>GPLGSVAAQKKKAQDEYGAASITILEGLEAVRKRPGMYIGSTGERGLHHLIWEVVDNAVDEAMAGYATTVNVVLLEDGGVEVADDGRGIPVATHASGIPTVDVVMTQLHAGGKFDSDAYAISGGLHGVGVSVVNALSTRLEVEIKRDGYEWSQVYEKSEPLGLKQGAPTKKTGSTVRFWADPAVFETTEYDFETVARRLQEMAFLNKGLTINLTDERVTQDEVVDEVVSDVAEAPKSASERAAESTAP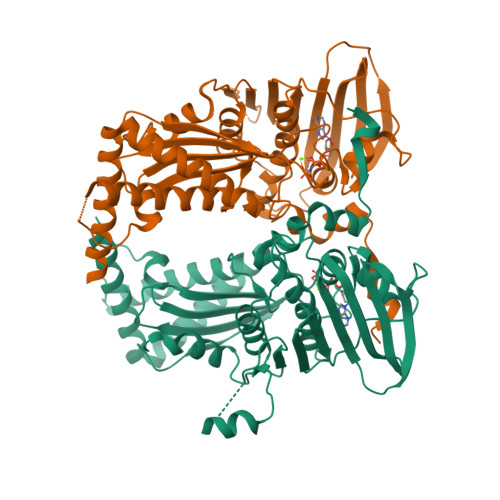HKVKSRTFHYPGGLVDFVKHINRTKNAIHSSIVDFSGKGTGHEVEIAMQWNAGYSESVHTFANTINTHEGGTHEEGFRSALTSVVNKYAKDRKLLKDKDPNLTGDDIREGLAAVISVKVSEPQFEGQTKTKLGNTEVKSFVQKVCNEQLTHWFEANPTDAKVVVNKAVSSAQARIAARKARELV[8x]> ATSDDWKSKAIYQLLTDRFGRADDSTSNCSNLSNYCGGTYEGITKHLDYISGMGFDAIWISPIPKNSDGGYHGYWATDFY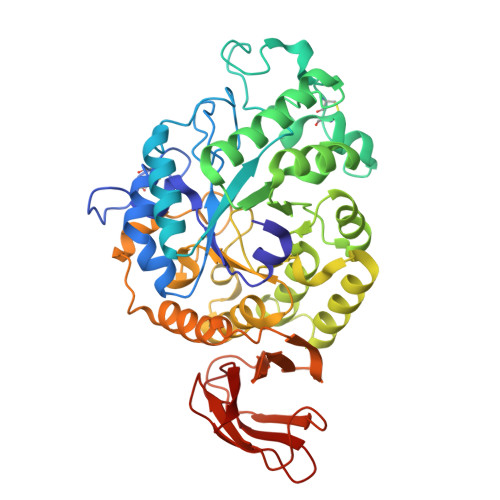QLNSNFGDESQLKALIQAAHERDMYVMLDVVANHAGPTSDGYSGYTFGDASLYHPKCTIDYNDQTSIEQCWVADELPDIDTENSDNVAILNDIVSGWVGNYSFDGIRIDTVKHIRKDFWTGYAEAAGVFATGEVFNGDPAYVGPYQKYLPSLINYPMYYALNDVFVSKSKGFSRISEMLGSNRNAFEDTSVLTTFVDNHDNPRFLNSQSDKALFKNALTYVLLGEGIPIVYYGSEQGFSGGADPANREVLWTTNYDTSSDLYQFIKTVNSVRMKSNKAVYMDIYVGDNAYAFKHGDALVVLNNYGSGSTNQVSFSVSGKFDSGASLMDIVSNITTTVSSDGTVTFNLKDGLPAIFTSA>MNSPIATVEVFTLTQPRKVPYLGALREGEVVNPNGYIVRKGNRTVYPTFDRSVLVRMTTEAGTVGWGETYGIVAPGAVAALINDLLAGFVIGRDASDPSAVYDDLYDMMRVRGYTGGFYVDALAA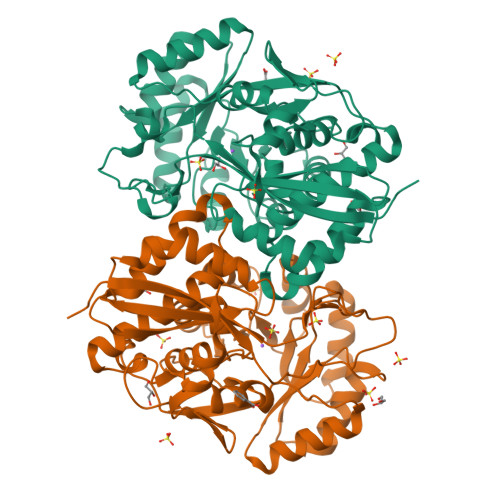LDIALWDIAGQEAGKSIRDLLGGGVDSFPAYVSGLPERTLKARGELAKYWQDRGFNAFKFATPVADDGPAAEIANLRQVLGPQAKIAADMHWNQTPERALELIAEMQPFDPWFAEAPVWTEDIAGLEKVSKNTDVPIAVGEEWRTHWDMRARIERCRIAIVQPEMGHKGITNFIRIGALAAEHGIDVIPHATVGAGIFLAASLQASSTLSMLKGHEFQHSIFEPNRRLLDGDMDCREGRYHLPSGPGLGVRPSEAALGLIERI[2x]> MTAISASVRPYDTIDLSSRAFWASSASQRESSFSELRAERPVSWHPPVEDALIQDPNDPGFWAVTRRADIVAVSRTNEVFLSGNGVLFENVPAELLEASQSFLAMDPPRHTKLRKLVSAAFTPRQVRRIEDSIKINAKGIVDELRMAGGGVDFVEHCAKELPIRTLSDMVGIPEADRERVAHAADALVSWADPRYLNGREPLAVLFENQMYLHQVAASLAAERRDRPGDDLFSALVNAEVDGDRLADADVAAFFVLLAVAGNDTTRQTISHGLKALTDFPSQKAWLLADFDTRIGTAVEELVRWATPVMTFRRTAAADFELGGQLIRAGEKVVMFYASGNWDEDAFCHPERLDLSRSPNPHVGFGGGGVHFCLGAHLARAQLRAIFGE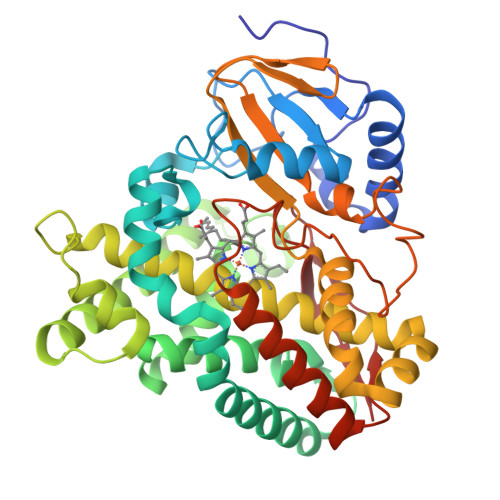LLVQLPDIQAGDPVYVPGNFVHAIRSMPCTF>MHHHHHHHHHHSSGLVPRGSHRILNLVKYDLYSIFKSPLTYLAILVVSSLIATQSILMANSMDNPKHIIVYGSVFAAAKWLLLIIGLMFVVKTITRDFSQGTIQLYMSKVKTRVGYIISKTISIILISILFALIHYVILIVVQASSNGKNLAFSKYVDNLWFFLIFLLFFGLFLFLITLASQKTAMIFSLGVFLVLIVPFIKPFITFIPRYGEKVLDAFDYIPFAYLTDKMISSNFDFSNWQWVISLGSIVIFFILNILYVAKKDI[2x];>[2x]MKLEHITKKYGSNVVLNDIDFDFGDSRIVGLIGKNGVGKTTVMKVMNGNIIKFDGKVDIDNADNIGFLIEHPKLYDNKSGLYNLKLFAQVLGKGFDKAYTDKIIDAFGMRPYIKKKVKKYSMGMKQKLAIAVSLMNKPKFLILDEPTNGMDPDGSIDVLTTIKSLVNELDMRILISSHKLEDIEL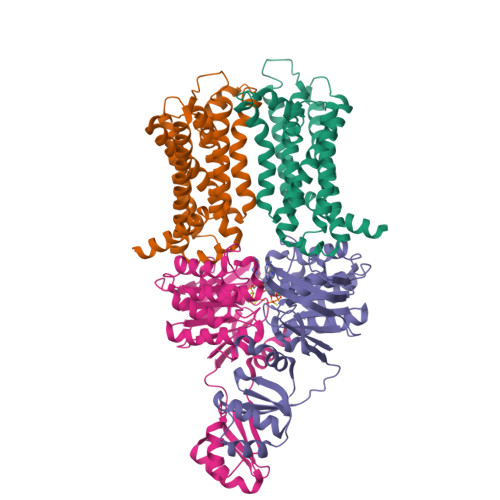ICDRAVFLRDGHFVQDVNMEEGVASDTTIVTVDHKDFDRTEKYLAEHFQLQNVDKADGHLMINAQKNYQVILKALSELDIYPKYIETRKSSLRDTYFNINQRGDK> MNANKQRQYNQLAHELRELQTNLQETTKQLDIMSKQCNENLVGQLGKVHGSWLIGSYIYYMEQMLG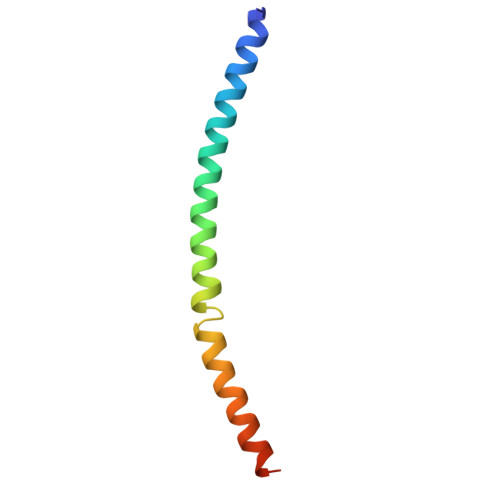KTQ5-bromo-4-chloro-1H-indol-3-yl 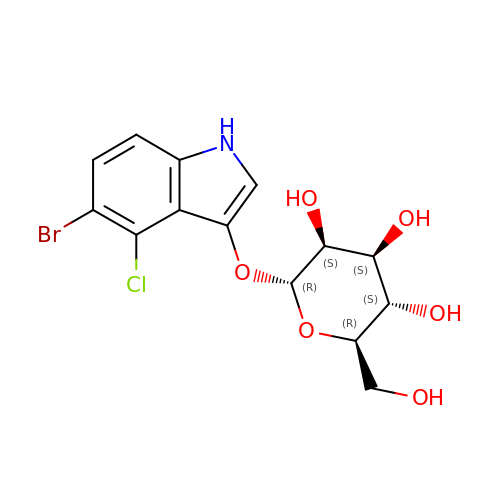alpha-D-mannopyranoside | C14 H15 Br Cl N O6 | OPIFSICVWOWJMJ-HAAGFXOZSA-N1,3-dimethylurea 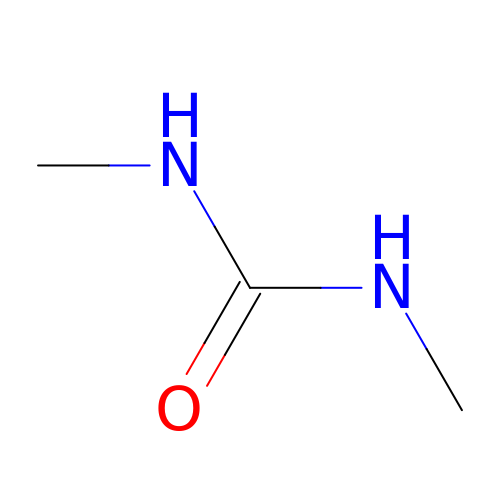| C3 H8 N2 O | MGJKQDOBUOMPEZ-UHFFFAOYSA-N> MKSSHHHHHHENLYFQSNATFSVTHARHMAAKVATDLRRMQR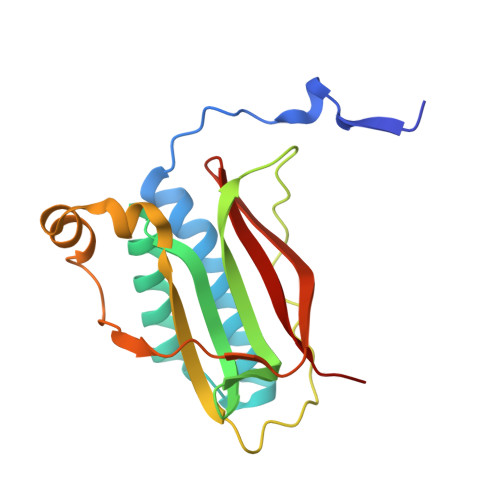FYGYPSDADIEAYEEELVVFLKAGYLGEVSYGFQKNNNWIEPTLRYTAGDLLGSGTDDDPGKIRPGKDVSGASFYSFMTYSSKYLNATQSEKDTALKDLPFKRVGAQSPGINGYLENDKTYSAGGRSLTRTSVRNFV> MRYPVTLTPAPEGGYMVSFV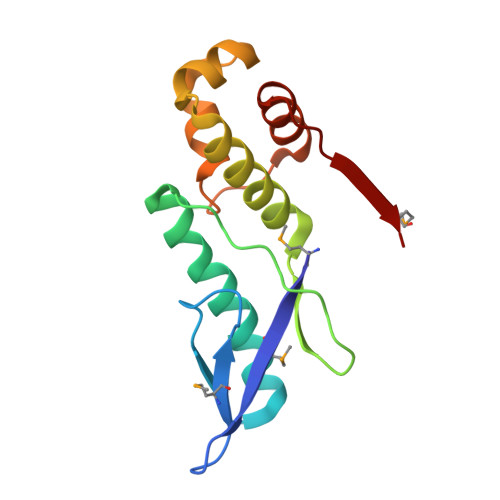DIPEALTQGETVAEAMEAAKDALLTAFDFYFEDNELIPLPSPLNSHDHFIEVPLSVASKVLLLNAFLQSEITQQELARRIGKPKQEITRLFNLHHATKIDAVQLAAKALGKELSLVMV Here, we provide the ligand/enzyme crystal complexes for one such PTP outlier: Arabidopsis thaliana Plant and Fungi Atypical Dual Specificity Phosphatase 1 (AtPFA-DSP1), herein unveiled as a regioselective and efficient phosphatase towards inositol pyrophosphate (PP-InsP) signaling molecules. Although the WPD loop is missing its canonical tripeptide motif, this structural element contributes to catalysis by assisting PP-InsP delivery into the catalytic pocket, for a choreographed exchange with phosphate reaction product. Subsequently, an intramolecular proton donation by PP-InsP substrate is posited to substitute functionally for the absent aspartate/glutamate general-acid. Additionally, we conclude that the hydrolyzed phosphate remains trapped as an enzyme-product complex, until it can be released in a prisoner exchange with another PP-InsP molecule; the latter process is assisted by the WPD loop.

The 5-InsP7 substrate is held in an 11.6 Å wide and 15.2 Å deep pocket by polar interactions between the 1-, 4-, 5β-, and 6-phosphates and multiple residues in the P-loop: Lys151, Arg152, Lys154, His155 and Arg156. These data also reveal that the His155 imidazole ring is flipped (180° χ2 angle changes) relative to its orientation in the Pi-bound crystal structures. We analogize such behavior by depicting His155 as a Janus residue, such that the catalytic core is overlooked by either of the two faces of the imidazole ring, depending upon the nature of the ligand: in this case, 5-InsP7 or Pi(A). The protonated Nε2 in His155 forms a polar contact with the PP-InsP substrate, and the Nδ1 forms a hydrogen bond with the hydroxyl group of Asp191, in which the carbonyl oxygen is further stabilized by Arg188. The 1- and 2-phosphates of 5-InsP7 also make multiple polar interactions with Lys186 in the α5-α6 loop. Gly118 and Lys120 from the WPD-loop make contributions to ligand binding with van der Waals interactions. Ser150, which replaces the catalytic cysteine, is located at the bottom of the ligand binding pocket and it helps to trap 5-InsP7 through its polar contact with one of the terminal oxygen atoms from the 5-β-phosphate moiety. We further noted that if a 1-β-phosphate were to be added to 5-InsP7, it would be solvent exposed, thereby rationalizing why 1,5-InsP8 is also actively hydrolyzed by this enzyme. Interestingly, catalytically productive binding of 1-InsP7, 2-InsP7 and 3-InsP7 is hindered by P-loop residues that would clash with either the axial 2-diphosphate or 2-monophosphate. This helps to explain why 1-InsP7, 2-InsP7 and 3-InsP7 are not efficient substrates for AtPFA-DSP1.

>[2x]GSFTEELHLIPPLNFSMVDNGIFRSGFPDSANFSFLQTLGLRSIIYLCPEPYPESNLQFLKSNGIRLFQFGIEGNKEPFVNIPDHKIRMALKVLLDEKNHPVLIHSKRGKHRTGCLVGCLRKLQKWCLTSIFDEYQRFAAAKARVSDQRFMEIFDVSSFSHIPMSFSCSIR>MNFFSLHPNVYATGRPKGLIGMLENVWVSNHTPGEGTLYLISGFSNYNGGVRFYETFTEHINQGGRVIAILGGSTSQRLSSRQVVEELLNRGVEVHIINRKRILHAKLYGTSNNLGESLVVSSGNFTGPGMSQNIEASLLLDNNTTQSMGFSWNDMISEMLNQNWHIHNMTNATDASPGWNLLYDERTTNLTLDETERVTLIVTLGHADTARIQAAPGTTAGQGTQYFWLSKDSYDFFPPLTIRNRRGTKATYSSLINMNYIDINYTDTQCRVT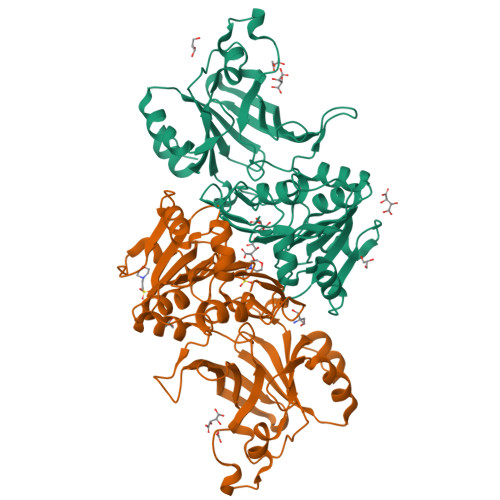FEAENNFDFRLGTGKLRYTGVAKSNDIAAITRVGDSDYELRIIKQGTPEHSQLDPYAVSFIGNRGKRFGYISNEEFGRIIGVTF[2x]>MSNEIPKPVAPAPDILRCAYAELVVTDLAKSRNFYVDVLGLHVSYEDENQIYLRSFEEFIHHNLVLTKGPVAALKAMAFRVRTPEDVDKAEAYYQELGCRTERRKDGFVKGIGDALRVEDPLGFPYEFFFETTHVERLHMRYDLYSAGELVRLDHFNQVTPDVPRGRKYLEDLGFRVTEDIQDDEGTTYAAWMHRKGTVEDTALTGGNGPRLHHVAFSTHEKHNIIQICDKMGALRISDRIERGPGRHGVSNAFYLYILDPDNH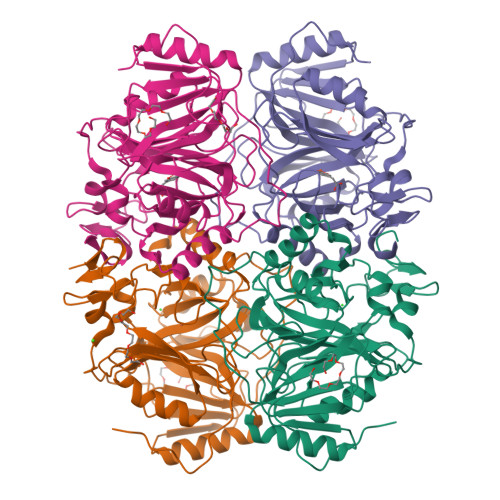RIEIYTQDYYTGDPDNPTITWNVHDNQRRDWWGNPVVPSWYTEASKVLDLDGNVQEIIERTDDSELEVTIGADGFSFTRAGDEDGSYHGQASKGFKLGNQL[4x]>[12x]MEKKITGYTTVDISQWHRKEHFEAFQSVAQCTYNQTVQLDITAFLKTVKKNKHKFYPAFIHILARLMNAHPEFRMAMKDGELVIWDSVH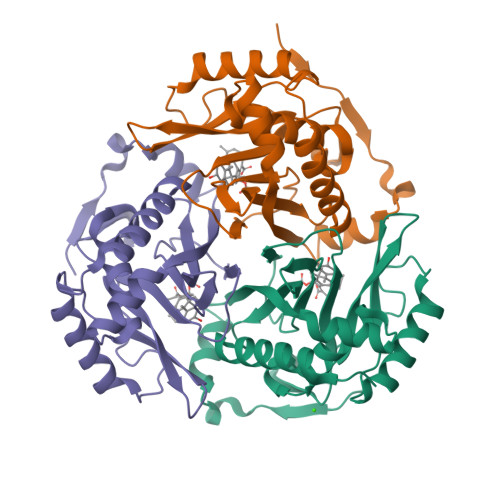PCYTVFHEQTETFSSLWSEYHDDFRQFLHIYSQDVACYGENLAYFPKGFIENMFFVSANPWVSFTSFDLNVANMDNFFAPVFTMGKYYTQGDKVLMPLAIQVHHAVCDGFHVGRMLNELQQYCDEWQGGA>[4x]MGKKMVVALGGNAILSNDASAHAQQQALVQTSAYLVHLIKQGHRLIVSHGNGPQVGNLLLQQQAADSEKNPAMPLDTCVAMTQGSIGYWLSNALNQELNKAGIKKQVATVLTQVVVDPADEAFKNPTKPIGPFLTEAEAKEAMQAGAIFKEDAGRGWRKVVPSPKPIDIHEAETINTLIKNDIITIS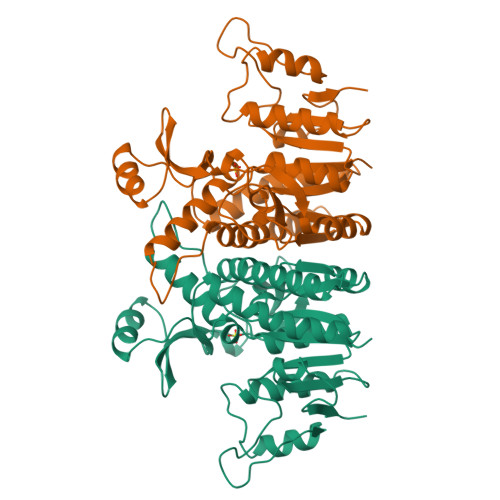CGGGGIPVVGQELKGVEAVIDKDFASEKLAELVDADALVILTGVDYVCINYGKPDEKQLTNVTVAELEEYKQAGHFAPGSMLPKIEAAIQFVESQPNKQAIITSLENLGSMSGDEIVGTVVTK>[4x]MAGARRLELGEALALGSGWRHVCWALLYAPDPGMLFGRIPLRYAILMQMRFDGRLGFPGGFVDTQDRSLEDGLNRELREE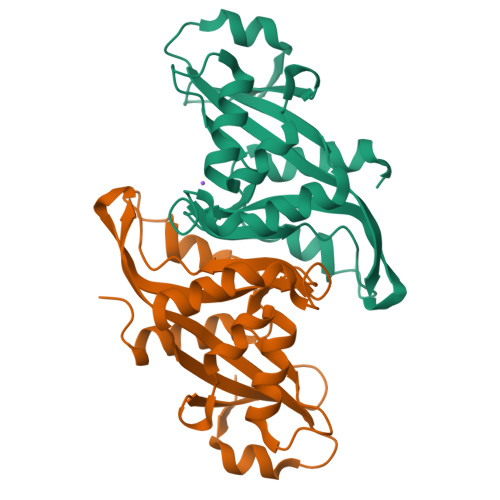LGEAAAAFRVERTDYRSSHVGSGPRVVAHFYAKRLTLEELLAVEAGATRAKDHGLEVLGLVRVPLYTLRDGVGGLPTFLENSFIGSAREQLLEALQDLGLLQSGSISGLKIPAHH> GTSTQTKAGSLTIVGTGIESIGQMTLQALSYIEAAAKVFYCVIDPATEAFILTKNKNCVDLYQYYDNGKSRLNTYTQMSELMVREVRKGLDVVGVFYGHPGVFVNPSHRALAIAKSEGYRARMLPGVSAEDCLFADLCIDPSNPGCLTYEASDFLIRDRPVSIHSHLVLFQVGCVGIADFNFTGFDNNKFGVLVDRLEQEYGAEHPVVHYIAAMMPHQ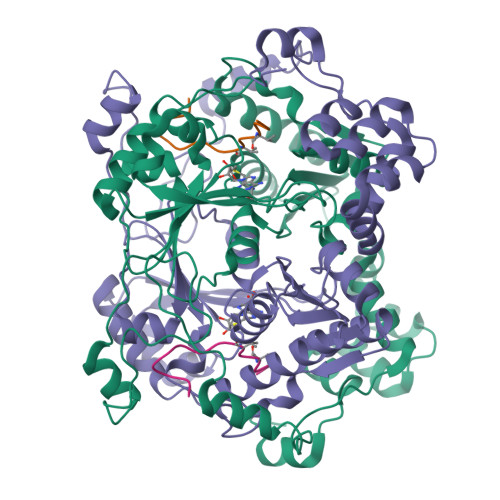DPVTDKYTVAQLREPEIAKRVGGVSTFYIPPKARKASNLDIIRRLELLPAGQVPDKKARIYPANQWEPDVPEVEPYRPSDQAAIAQLADHAPPEQYQPLATSKAMSDVMTKLALDPKALADYKADHRAFAQSVPDLTPQERAALELGDSWAIRCAMKNMPSSLLDAARESGEEASQNGFPWVIVFGVIGVIG;> FPWVIVFGVIGVIG2-{(R)-(3-aminophenyl)[2-(piperidin-1-yl)ethoxy]methyl}thieno[3,2-b]pyridine-7-carboxylic acid | C22 H25 N3 O3 S | 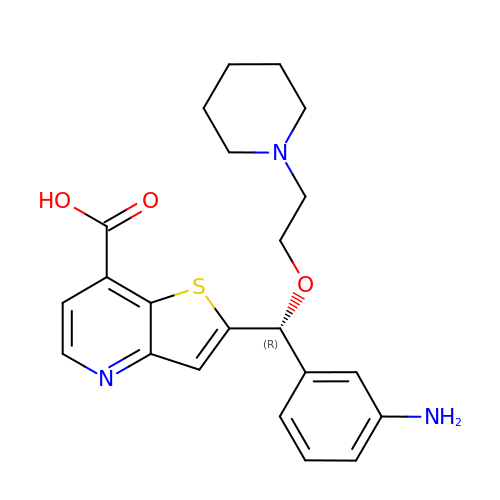FTKYSFLMVOPKTH-HXUWFJFHSA-N4-[[(1~{S})-2-[(~{E})-3-[5-chloranyl-2-(1,2,3,4-tetrazol-1-yl)phenyl]prop-2-enoyl]-5-[(3~{S})-3-ethoxycarbonylpiperidin-1-yl]carbonyl-3,4-dihydro-1~{H}-isoquinolin-1-yl]carbonylamino]benzoic acid | C36 H34 Cl N7 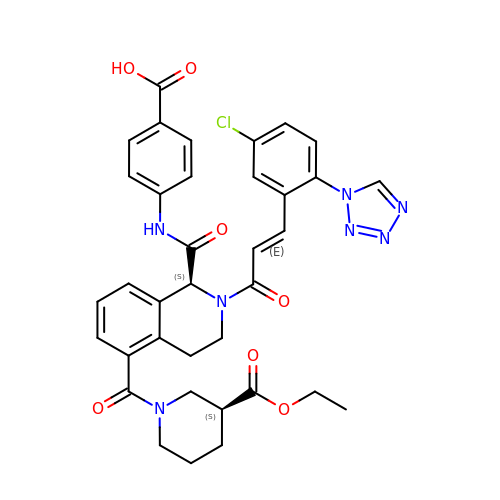O7 | ZDVKEWAKPHMOKV-WTBNABMMSA-N>[5x]GSHMVMNTHPYQSEAVSDVWSLSKTSMTFQPKKASLQPLTISLDELFSSRGEFISVGGNGRMSHKEAILLGLRYKKLYNQARVKYSL;>[5x]SVTVKRIIDNTVIVPKLPANEDPVEYPADYFRKSKEIPLYINTTKSLSDLRGYVYQGLKSGNVSIIHVNSYLYGALKDIRGKLDKDWSSFGINIGKAGDTIGIFDLVSLKALDGVLPDGVSDASRTSADDKWLPLYLLGLYRVGRTQMPEYRKKLMDGLTNQCKMINEQFEPLVPEGRDIFDVWGNDSNYTKIVAAVDMFFHMFKKHECASFRYGTIVSRFKDCAALATFGHLCKITGMSTEDVTTWILNREVADEMVQMMLPGQEIDKADSYMPYLIDFGLSSKSPYSSVKNPAFHFWGQLTALLLRSTRARNARQPDDIEYTSLTTAGLLYAYAVGSSADLAQQFCVGDNKYTPDDSTGGLTTNAPPQGRDVVEWLGWFEDQNRKPTPDMMQ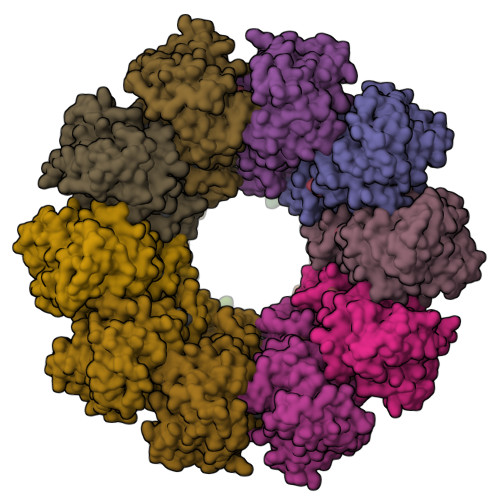YAKRAVMSLQGLREKTIGKYAKSEFDK>AGPQLDVSCFAHDKNIGSRTEQLSV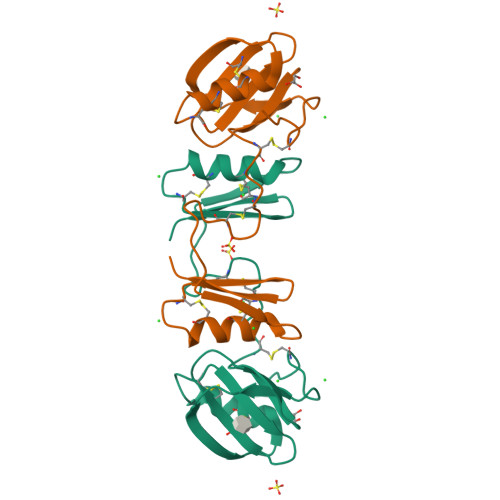VHVASAQDCMKECQALPTCSHFTYNKNSKKCHLKAGAPEFYTYTGDMTGPRSCEHNCSDACWMDGNNPLAVWDYSGQPPALCWAACMGTPGCDLYTFQGMTCKLYSQTSSKRA[2x]>MAKNIQAIRGMNDYLPGETAIWQRIEGTLKNVLGSYGYSEIRLPIVEQTPLFKRAIGEVTDVVEKEMYTFEDRNGDSLTLRPEGTAGCVRAGIEHGLLYNQEQRLWYIGPMFRHERPQKGRYRQFHQLGCEVFGLQGPDIDAELIMLTARWWRALGISEHVTLELNSIGSLEARANYRDALVAFLEQHKEKLDEDCKRRMYTNPLRVLDSKNPEVQALLNDAPALGDYLDEESREHFAGLCKLLESAGIAYTVNQRLVRGLDYYNRTVFEWVTNSLGSQGTVCAGGRYDGLVEQLGGRATPAVGFAMGLERLVLLVQAVNPEFKADPVVDIYLVASGADTQSAAMALAERLRDELPGVKLMTNHGGGNFKKQFARADKWGAR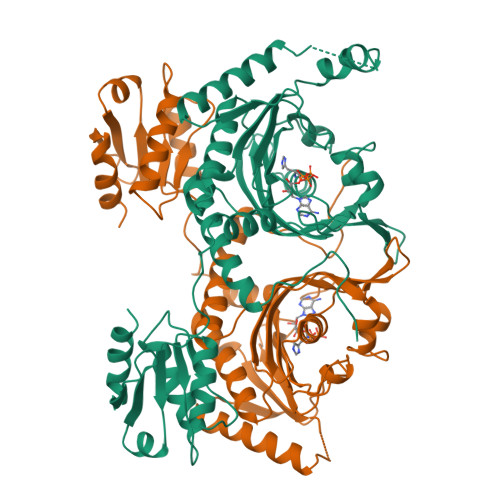VAVVLGESEVANGTAVVKDLRSGEQTAVAQDSVAAHLRTLLG[4x]> PMTKVLKADDINKAISAFKDPGTFDYKR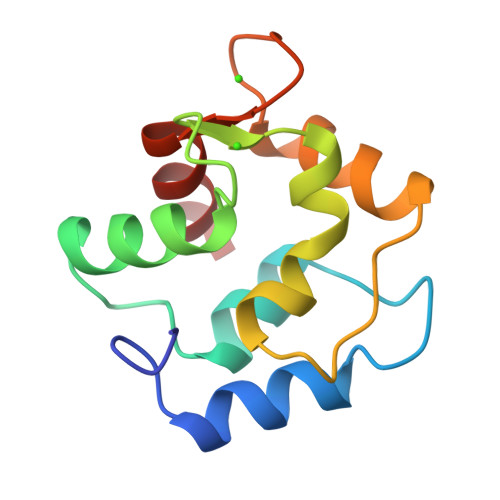FFHLVGLKGKTDAQVKEVFEILDKDQSGFIEEEELKGVLKGFSAHGRDLNDTETKALLAAGDSDHDGKIGADEFAKMVAQA>MWKRSEQMKIKSGKCNMAAAMETEQLGVEIFETADCEENIESQDRPKLEPFYVERYSWSQLKKLLADTRKYHGYMMAKAPHDFMFVKRNDPDGPHSDRIYYLAMSGENRENTLFYSEIPKTINRAAVLMLSWKPLLDLFQATLDYGMYSREEELLRERKRIGTVGIASYDYHQGSGTFLFQAGSGIYHVKDGGPQGFTQQPLRPNLVETSCPNIRMDPKLCPADPDWIAFIHSNDIWISNIVTREERRLTYVHNELANMEEDARSAGVATFVLQEEFDRYSGYWWCPKAETTPSGGKILRILYEENDESEVEIIHVTSPMLETRRADSFRYPKTGTANPKVTFKMSEIMIDAEGRIIDVIDKELIQPFEILFEGVEYIARAGWTPEGKYAWSILLDRSQTRLQIVLISPELFIPVEDDVMERQRLIESVPDSVTPLIIYEETTDIWINIHDIFHVFPQSHEEEIEFIFASECKTGFRHLYKITSILKESKYKRSSGGLPAPSDFKCPIKEEIAITSGEWEVLGRHGSNIQVDEVRRLVYFEGTKDSPLEHHLYVVSYVNPGEVTRLTDRGYSHS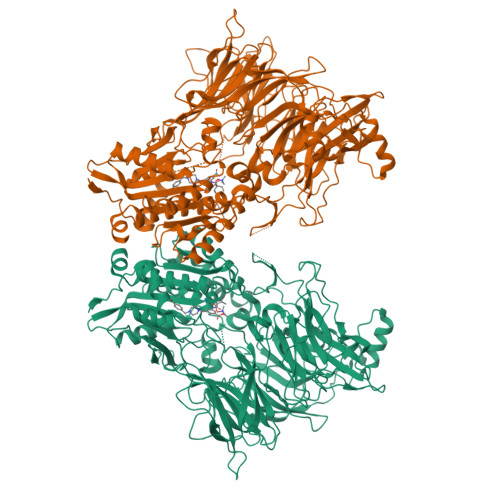CCISQHCDFFISKYSNQKNPHCVSLYKLSSPEDDPTCKTKEFWATILDSAGPLPDYTPPEIFSFESTTGFTLYGMLYKPHDLQPGKKYPTVLFIYGGPQVQLVNNRFKGVKYFRLNTLASLGYVVVVIDNRGSCHRGLKFEGAFKYKMGQIEIDDQVEGLQYLASRYDFIDLDRVGIHGWSYGGYLSLMALMQRSDIFRVAIAGAPVTLWIFYDTGYTERYMGHPDQNEQGYYLGSVAMQAEKFPSEPNRLLLLHGFLDENVHFAHTSILLSFLVRAGKPYDLQIYPQERHSIRVPESGEHYELHLLHYLQENLGSRIAALKVI[2x]>[2x]MNACPHSDTLTIDPMITDLAGETSRLRAAGPLTRIDLLGVPALAVTGHTLARQLLTDTRLVKDINAWSLWQSGTVTRQWPLIGMIDVDRSMFTVDGPEHRRLRIKTTQALTRRRLDALKPTIERYVAELLDDLERAGADGAVVDLKSVFAYPLPMRVISALMGVPSEDQEQLLTWYKAFFSILTPQDERLRVIDEMHGYFTEMVRRKTAEPGDDLTSALIYATDGETPLTEEEVIGNLQALVAAGHETTVSLILTAVRALLSHPEQLRLVRDGEIGWETAIEETLRWDGPVIHLLMRFATEDIDLGDAVIPRGEGVVMSYRAIGRDITVHGADADDFDITRATAARHISFGHGPHICPGAALARLEAAIALPALFTRFPHLHPALPLDQIPNLPVLTQNDLSHFPIHLG

CYP154C5 from Nocardia farcinica is a P450 monooxygenase able to hydroxylate a range of steroids with high regio‐ and stereoselectivity at the 16α‐position. Recently, the crystal structure of CYP154C5, a cytochrome P450 monooxygenase from Nocardia farcinica, was elucidated in the presence of four steroid substrates. This enzyme catalyzes the highly regio‐ and stereoselective hydroxylation of different pregnans and androstans producing exclusively the corresponding 16α‐hydroxylated products. The active site pocket of CYP154C5 forms a hydrophobic “tube” with two opposite polar regions at both ends. These polar regions are occupied by Gln239 and Gln398 forming hydrogen bond interactions with the hydroxy or ketone functionalities of steroids at positions C3 (via water molecules) and C17.

Moreover, exclusive 15α‐hydroxylation was observed for wild‐type CYP154C5 in the conversion of 5α‐androstan‐3‐one, lacking an oxy‐functional group at C17. To gain structural insight into the altered regioselectivity of wild‐type CYP154C5 in the conversion of 11, the P450 was co‐crystallized with this steroid. The overall structure of CYP154C5 is very similar to the previously determined CYP154C5 structures with Cα‐RMSD values of 0.20–0.37. The electron density of the ligand and the derived model indicate that 5α‐androstan‐3‐one binds in a similar position as androstenedione and testosterone (5), the latter being hydroxylated in 16α position by wild‐type CYP154C5. Interestingly, however, C15 of steroids 4, 5 and 11 in the corresponding crystal structures of CYP154C5 are in a similar position as C16 of pregnenolone and progesterone (3), which are also hydroxylated in 16α position by wild‐type CYP154C5. Hence, the crystal structure alone cannot explain the observed hydroxylation of 5α‐androstan‐3‐one in 15α‐position. Therefore, MD simulations (10 trajectories of 22 ns each) of the compound I state of the CYP154C5 structure with 11 bound in the active site have been performed with scoring of NACs. This way, predicted NAC percentages of 0.31 % for C15 and 15.8 % for C16 were obtained.>MRGSHHHHHHGMASHMATEQTAITRATFDEVILPVYAPADFIPVKGKGSRVWDQQGKEYIDFAGGIAVTALGHCHPALVEALKSQGETLWHTSNVFTNEPALRLGRKLIDATFAERVLFMNSGTEANETAFKLARHYACVRHSPFKTKIIAFHNAFHGRSLFTVSVGGQPKYSDGFGPKPADIIHVPFNDLHAVKAVMDDHTCAVVVEPIQGEGGVQAATPEFLKGLRDLCDEHQALLVFDEVQCGMGRTGDLFAYMHYGVTPDILTSAKALGGGFPVSAMLTTQEIASAFHVGSHGSTYGGNPLACAVAGAAFDIINTPEVLQGIHTKRQQFVQHLQA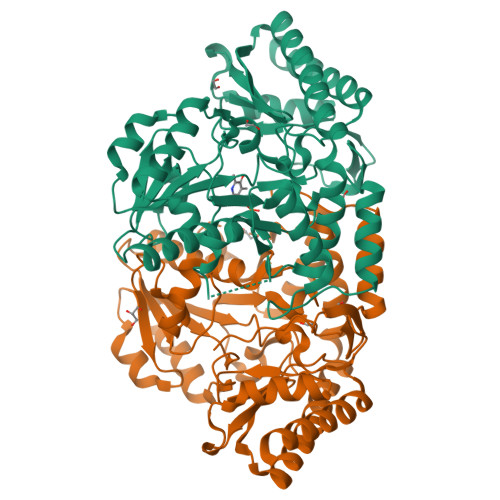IDEQFDIFSDIRGMGLLIGAELKPKYKGRARDFLYAGAEAGVMVLNAGADVMRFAPSLVVEEADIHEGMQRFAQAVGKVVA[2x]> GEVVDCHLSDMLQQLHSVNASKPSERGLVRQEEAEDPACIPIFWVSKWVDYSDKYGLGYQLCDNSVGVLFNDSTRLILYNDGDSLQYIERDGTESYLTVSSHPNSLMKKITLLKYFRNYMSEHLLKAGANITPREGDELARLPYLRTWFRTRSAIILHLSNGSVQINFFQDHTKLILCPLMAAVTYIDEKRDFRTYRLSLLE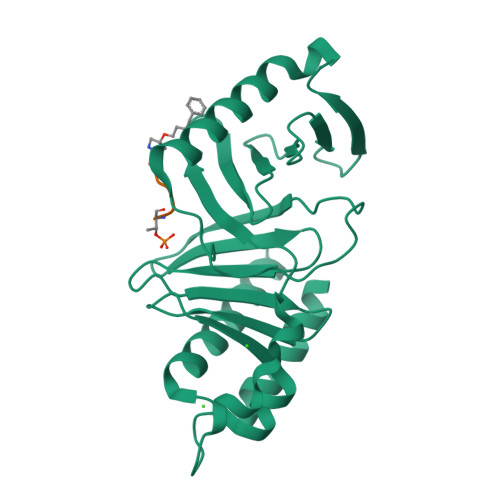EYGCCKELASRLRYARTMVDKLLSSRSASNRLKAS>HHHHHHMSAIENFDAHTPMMQQYLRLKAQHPEILLFYRMGDFYELFYDDAKRASQLLDISLTKRGASAGEPIPMAGIPYHAVENYLAKLVNQGESVAICEQIGDPATSKGPVERKVVRIVTPGTISDEALLQERQDNLLAAIWQDSKGFGYATLDISSGRFRLSEPADRETMAAELQRTNPAELLYAEDFAEMSLIEGRRGLRRRPLWEFEIDTARQQLNLQFGTRDLVGFGVENAPRGLCAAGCLLQYAKDTQRTTLPHIRSITMEREQDSIIMDAATRRNLEITQNLAGGAENTLAS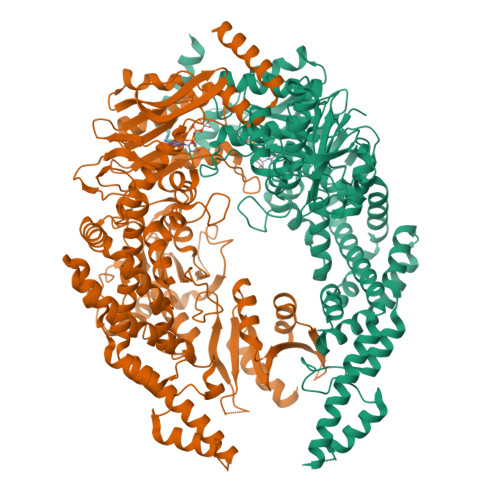VLDCTVTPMGSRMLKRWLHMPVRDTRVLLERQQTIGALQDFTAGLQPVLRQVGDLERILARLALRTARPRDLARMRHAFQQLPELRAQLETVDSAPVQALREKMGEFAELRDLLERAIIDTPPVLVRDGGVIASGYNEELDEWRALADGATDYLERLEVRERERTGLDTLKVGFNAVHGYYIQISRGQSHLAPINYMRRQTLKNAERYIIPELKEYEDKVLTSKGKALALEKQLYEELFDLLLPHLEALQQSASALAELDVLVNLAERAYTLNYTCPTFIDKPGIRITEGRHPVVEQVLNEPFIANPLNLSPQRRMLIITGPNMGGKSTYMRQTALIALMAYIGSYVPAQKVEIGPIDRIFTRVGAADDLASGRSTFMVEMTETANILHNATEYSLVLMDEIGRGTSTYDGLSLAWACAENLANKIKALTLFATHYFELTQLPEKMEGVANVHLDALEHGDTIAFMHSVQDGAASKSYGLAVAALAGVPKEVIKRARQKLRELESIS[2x]> MTLEKFVDALPIPDTLKPVQQSKEKTYYEVTMEECTHQLHRDLPPTRLWGYNGLFPGPTIEVKRNENVYVKWMNNLPSTHFLPIDHTIHHSDSQHEEPEVKTVVHLHGGVTPDDSDGYPEAWFSKDFEQTGPYFKREVYHYPNQQRGAILWYHDHAMALTRLNVYAGLVGAYIIHDPKEKRLKLPSDEYDVPLLITDRTINEDGSLFYPSAPENPSPSLPNPSIVPAFCGETILVNGKVWPYLEVEPRKYRFRVINASNTRTYNLSLDNGGDFIQIGSDGGLLPRSVKLNSFSLAPAERYDIIIDFTAYEGESIILANSAGCGGDVNPETDANIMQFRVTKPLAQKDESRKPKYLASYPSVQHERIQNIRTLKLAGTQDEYGRPVLLLNNKRWHDPVTETPKVGTTEIWSIINPTRGTHPIHLHLVSFRVLDRRPFDIARYQESGELSYTGPAVPPPPSEKGWKDTIQAHAGEVLRIAATFGPYSGRYVWHCHILEHEDYDMMRPMDITDPHK

Spore coat protein A (CotA) is a protein isolated from the bacterium Bacillus subtilis. It is able to oxidize specific laccase substrates and is characterized as a typical laccase with one mononuclear copper centre (T1 copper) and one trinuclear centre (TNC) comprised of one T2 copper and two T3 coppers. Substrate oxidation occurs at the T1 binding pocket and the electrons are then shuttled to the TNC, where the reduction of dioxygen occurs. The overall structure of CotA comprises three cupredoxin-type domains, characterized by a Greek-key β-barrel topology, which is similar to other multi-copper oxidases.

Here, we report the crystal structure of CotA complexed with a nonphenolic substrate, 2,2-azinobis-(3-ethylbenzothiazoline-6-sulfonate) (ABTS). The ABTS molecule unexpectedly binds to the positively charged hole in the protein. In the structure of the CotA–ABTS complex, ABTS was observed sitting within the hole. The novel binding site was approximately 26 Å away from the T1 binding pocket and was near the exit of the water channel. The ABTS molecule passed through the hole in a linear shape and interacted with adjacent residues by hydrophobic contacts: Ile408, Leu431, Ile366, Ala478 and Trp463. The sulfonate moiety at one end of ABTS formed two hydrogen bonds to the guanidyl group of Arg476 (Arg476 NH1–O48 = 3.1 Å, Arg476 NH2–O49 = 3.1 Å), and the sulfonate moiety at the other end of ABTS formed a hydrogen bond to Ser360 (Ser360 N–O45 = 3.1 Å). The thiazoline ring of ABTS was almost buried in the hole, and the two sulfonate moieties of ABTS were exposed to the external environment. In the CotA–ABTS complex, conformational changes were observed upon substrate binding. A 310-helical fragment composed of residues 359–362 was dissolved and the side chains of Arg429 and Arg146 were rotated by about 40 and 120°, respectively, providing more space for ABTS binding. In our study, the ABTS passed through the hole in a linear shape; the B factor of ABTS was 35.6 Å2 and it had full occupancy.>[2x]MFEQRVNS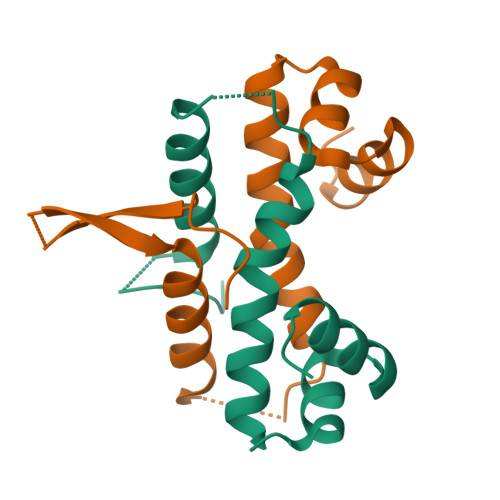DVLTVSTVNSQDQVTQKPLRDSVKQALKNYFAQLNGQDVNDLYELVLAEVEQPLLDMVMQYTRDNQTRAALMMGINRGTLRKKLKKYGMN>[4x]MPKETPSKAAADALSDLEIKDSKSNLNKELETLREENRVKSDMLKEKLSKDAENHKAYLKSHQVHRHKLKEMEKEEPLLNEDKERTVLFPIKYHEIWQAYKRAEASFWTAEEIDLSKDIHDWNNRMNENERFFISRVL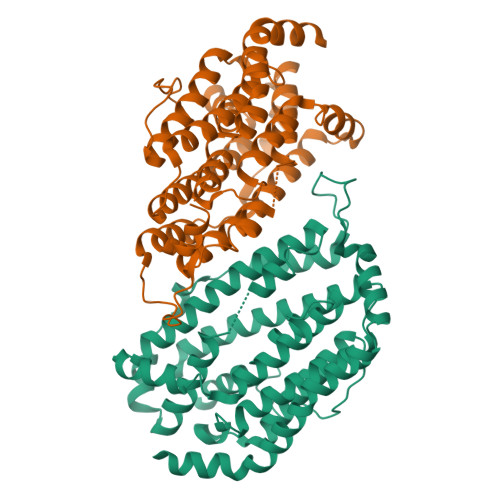AFFAASDGIVNENLVENFSTEVQIPEAKSFYGFQIMIENIHSETYSLLIDTYIKDPKESEFLFNAIHTIPEIGEKAEWALRWIQDADALFGERLVAFASIEGVFFSGSFASIFWLKKRGMMPGLTFSNELICRDEGLHTDFACLLFAHLKNKPDPAIVEKIVTEAVEIEQRYFLDALPVALLGMNADLMNQYVEFVADRLLVAFGNKKYYKVENPFDFMENISLAGKTNFFEKRVSDYQKAGVMSKSTKQEAGAFTFNEDF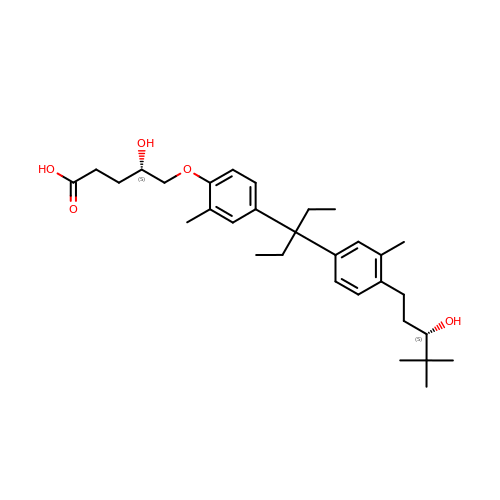(4S)-4-hydroxy-5-[4-(3-{4-[(3S)-3-hydroxy-4,4-dimethylpentyl]-3-methylphenyl}pentan-3-yl)-2-methylphenoxy]pentanoic acid | C31 H46 O5 | YAAVVZVAZRPBGF-XCZPVHLTSA-N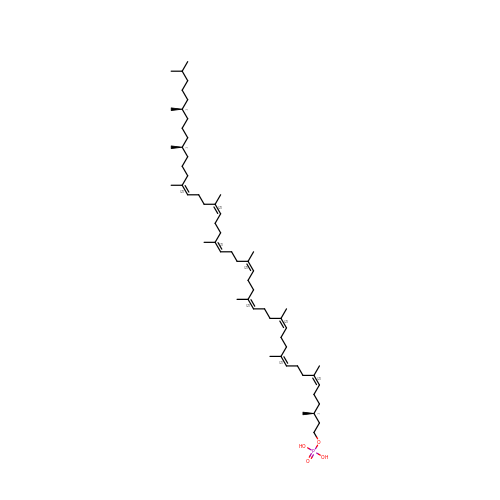[(3S,6Z,10Z,14Z,18Z,22Z,26Z,30Z,34Z,39S,43S)-3,7,11,15,19,23,27,31,35,39,43,47-dodecamethyloctatetraconta-6,10,14,18,22,26,30,34-octaenyl] dihydrogen phosphate | C60 H107 O4 P | XTTHNPQIJYVHIB-WHVVPYAWSA-N>[6x]MPNVDMPLSQLQDYKPELTNETDFDLFWDNAKALSNQKPLHAQVNLVQDYPLKSISIYDVVYDGADGTPIHGWYVTPKGEHQPGSLPVLVKYHGYSGNRG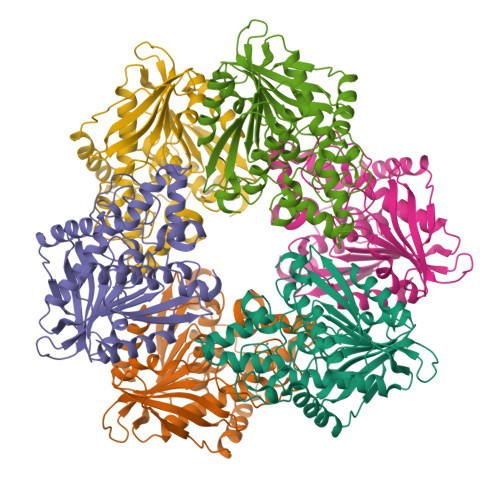YPNELLQWASMGMAALAIDVRGQGGVTPDRAEYPQGGIPGWMTLGILDPASYYYKQVYLDCIRALDFVCSREEVDASRIAVYGGSQGGGLALAAAGLDSRPKLALPVFPFLCHFRRSVEIHASGPYVEIKNWFRRYDPEHRQEEQVYRTLSYFDGMNMASRIKARTLMAITLQDITCPPSTCFAAYNHLAGPKEVRLYHDYGHEGLPFHEEAMMRFIEAYL>[2x]GSSSLQRLEELFRRYKDEREDAILEEGMERFCNDLCVDPTEFRVLLLAWKFQAATMCKFTRKEFFDGCKAISADSIDGICARFPSLLTEAKQEDKFKDLYRFT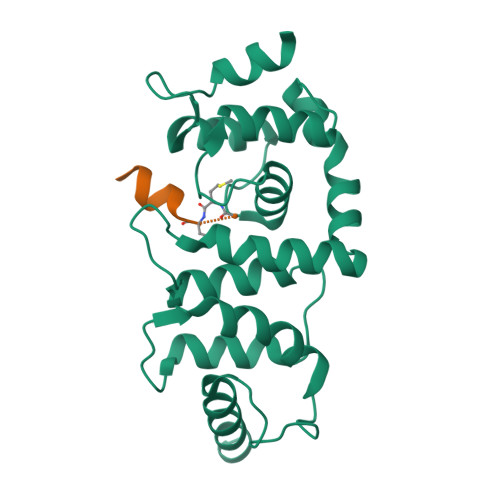FQFGLDSEEGQRSLHREIAIALWKLVFTQNNPPVLDQWLNFLTENPSGIKGISRDTWNMFLNFTQVIGPDLSNYSEDEAWPSLFDTFVEWEMERRKREGEGRGALSSGPEGLCPEEQT;>[2x]MLTLASKLKRDDGLKGSRTAATASD>[2x]SLEA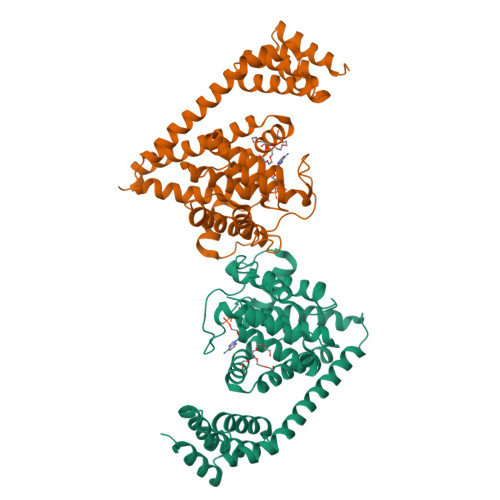RAALNQALEMKRQGKREKAQKLFMHALKMDPDFVDALTEFGIFSEEDKDIIQADYLYTRALTISPYHEKALVNRDRTLPLVEEIDQRYFSIIDSKVKKVMSIPKGNSALRRVMEETYYHHIYHTVAIEGNTLTLSEIRHILETRYAVPGKSLEEQNEVIGMHAAMKYINTTLVSRIGSVTISDVLEIHRRVLGYVDPVEAGRFRTTQVLVGHHIPPHPQDVEKQMQEFVQWLNSEEAMNLHPVEFAALAHYKLVYIHPFIDGNGRTSRLLMNLILMQAGYPPITIRKEQRSDYYHVLEAANEGDVRPFIRFIAKCTETTLDTLLFATTEYSVALPEAQP>MTRLDSVERAVADIAAGKAVIVIDDEDRENEGDLIFAAEKATPEMVAFMVRYTSGYLCVPLDGAICDRLGLLPMYAVNQDKHGTAYTVTVDARNGIGTGISASDRATTMRLLADPTSVADDFTRPGHVVPLRAKDGGVLRRPGH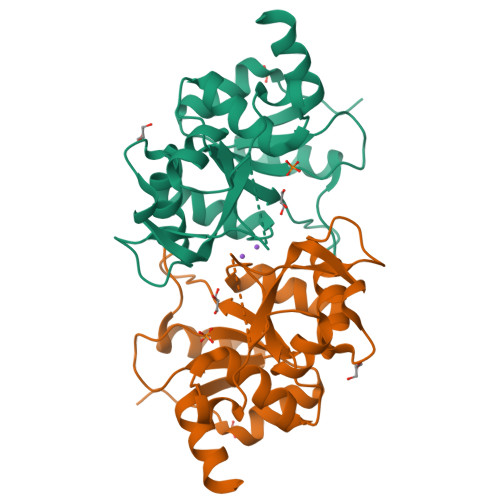TEAAVDLARMAGLQPAGAICEIVSQKDEGSMAHTDELRVFADEHGLALITIADLIEWRRKHE[2x]>[2x]MKKGHHHHHHGSERTGTQPLGVQGLTEEQRMMIRELMDAQMKTFDTTFSHFKNFRLPGVLSSGCELPESLQAPSREEAAKWSQVRKDLCSLKVSLQLRGEDGSVWNYKPPADSGGKEIFSLLPHMADMSTYMFKGIISFAKVISYFRDLPIEDQISLLKGAAFELCQLRFNTVFNAETGTWECGRLSYCLEDTAGGFQQLLLEPMLKFHYMLKKLQLHEEEYVLMQAISLFSPDRPGVLQH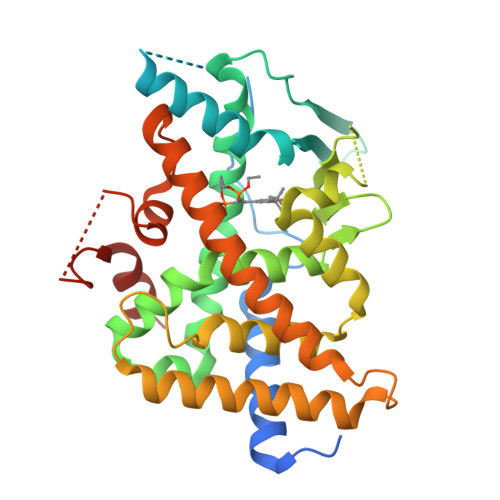RVVDQLQEQFAITLKSYIECNRPQPAHRFLFLKIMAMLTELRSINAQHTQRLLRIQDIHPFATPLMQELFGITGSLVPRGSSSHSSLTERHKILHRLLQEGSPS> AQLREYHIAAQLEDWDYNPQPEELSRLSESDLTFKKIVYREYELDFKQEKPRDALSGLLGPTLRGEVGDSLIIYFKNFATQPVSIHPQSAVYNKWSEGSSYSDGTSDVERLDDAVPPGQSFKYVWNITAEIGPKKADPPCLTYAYYSHV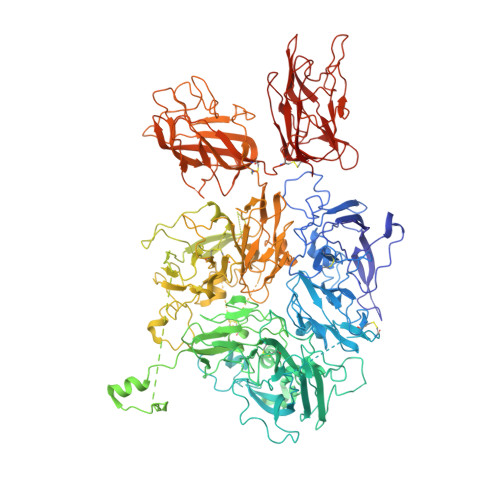NMVRDFNSGLIGALLICKEGSLNANGSQKFFNREYVLMFSVFDESKNWYRKPSLQYTINGFANGTLPDVQACAYDHISWHLIGMSSSPEIFSVHFNGQTLEQNHYKVSTINLVGGASVTADMSVSRTGKWLISSLVAKHLQAGMYGYLNIKDCGNPDTLTRKLSFRELMKIKNWEYFIAAEEITWDYAPEIPSSVDRRYKAQYLDNFSNFIGKKYKKAVFRQYEDGNFTKPTYAIWPKERGILGPVIKAKVRDTVTIVFKNLASRPYSIYVHGVSVSKDAEGAIYPSDPKENITHGKAVEPGQVYTYKWTVLDTDEPTVKDSECITKLYHSAVDMTRDIASGLIGPLLVCKHKALSVKGVQNKADVEQHAVFAVFDENKSWYLEDNIKKYCSNPSAVKKDDPKFYKSNVMYTLNGYASDRTEVLRFHQSEVVQWHLTSVGTVDEIVPVHLSGHTFLSKGKHQDILNLFPMSGESATVTMDNLGTWLLSSWGSCEMSNGMRLRFLDANYDDEDEGNEEEEEDDGDIFADIFIPSEVVKKKEEVPVNFVPDPESDALAKELGLIDDEGNPIIQPRREQTEDDEEQLMKASMLGLRSFKGSVAEEELKHTALALEEDAHASDPRIDSNSARNPDDIAGRYLRTINRGNKRRYYIAAEEVLWDYSPIGKSQVRSRAAKTTFKKAIFRSYLDDTFQTPSTGGEYEKHLGILGPIIRAEVDDVIEIQFKNLASRPYSLHAHGLLYEKSSEGRSYDDKSPELFKKDDAIMPNGTYTYVWQVPPRSGPTDNTEKCKSWAYYSGVNPEKDIHSGLIGPILICQKGMIDKYNRTIDIREFVLFFMVFDEEKSWYFPKSDKSTCEEKLIGVQSLHTFPAINGIPYQLQGLTMYKDENVHWHLLNMGGPKDIHVVNFHGQTFTEEGREDNQLGVLPLLPGTFASIKMKPSKIGTWLLETEVGENQERGMQALFTVIDKDCKLPMGLASGIIQDSQISASGHVGYWEPKLARLNNTGKYNAWSIIKKEHEHPWIQIDLQRQVVITGIQTQGTVQLLQHSYTVEYFVTYSEDGQNWITFKGRHSETQMHFEGNSDGTTVKENHIDPPIIARYIRLHPTKFYNRPTFRIELLGCEVEGCSVPLGMESGAIKNKEITASSYKKTWWSSWEPFLARLNLEGGTNAWQPEVNNKDQWLQIDLQHLTKITSIITQGATSMTTSMYVKTFSIHYTDDNSTWKPYLDVRTSMEKVFTGNINSDGHVKHFFKPPILSRFIRIIPKTWNQYIALRIELFGCEVF> VEFNTDVLDAADKKNIDFTRFSEAGYVLPGQYLLDVIVNGQSISPASLQISFVEPQSSGDKAEKKLPQACLTSDMVRLMGLTAESLDKVVYWHDGQCADFHGLPGVDIRPDTGAGVLRINMPQARLEYSDATWLPPSRWDDGIPGLMLDYNLNGTVSRNYQGGDSHQFSYNGTVGGNLGPWRLRADYQGSQEQSRYNGEKTTNRNFTWSRFYLFRAIPRWRANLTLGENNINSDIFRSWSYTGASLESDDRMLPPRLRGYAPQITGIAETNARVVVSQQGRVLYDSMVPAGPFSIQDLDSSVRGRLDVEVIEQNGRKKTFQVDTASVPYLTRPGQVRYKLVSGRSRGYGHETEGPVFATGEASWGLSNQWSLYGGAVLAGDYNALAAGAGWDLGVPGTLSADITQSVARIEGERTFQGKSWRLSYSKRFDNADADITFAGYRFSERNYMTMEQYLNARYRNDYSSREKEMYTVTLNKNVADWNTSFNLQYSRQTYWDIRKTDYYTVSVNRYFNVFGLQGVAVGLSASRSKYLGRDNDSAYLRISVPLGTGTASYSGSMSNDRYVNMAGYTDTFNDGLDSYSLNAGLNSGGGLTSQRQINAYYSHRSPLANLSANIASLQKGYTSFGVSASGGATITGKDAALHAGGMSGGTRLLVDTDGVGGVPVDGGQVVTNRWGTGVVTDISSYYRNTTSVDLKRLPDDVEATRSVVESALTEGAIGYRKFSVLKGKRLFAILRLADGSQPPFGASVTSEKGRELGMVADEGLAWLSGVTPGETLSVNWDGKIQCQVNVPETAISDQQLLLPCTPQK;> AVSLDRTRAVFDGSEKSMTLDISNDNKQLPYLAQAWIENENQEKIITGPVIATPPVQRLEPGAKSMVRLSTTPDISKLPQDRESLFYFNLREIPPRSEKANVLQIALQTKIKLFYRPAAIKTRPNEVWQDQLILNKVSGGYRIENPTPYYVTVIGLGGSEKQAEEGEFETVMLSPRSEQTVKSANYNTPYLSYINDYGGRPVLSFICNGSRCSVKKEK;> MIRLSLFISLLLTSVTVLADVQINIRGHVYIPPCTINNGQNIVVDFGNINPEHVDNSRGEVTKTISISCPYKSGSLWIKVTGNTMGGGQNNVLATNITHFGIALYQGKGMSTPLTLGNGSGNGYRVTAGLDTARSTFTFTSVPFRNGSGILNGGDFRTTASMSMIYN;> MKKWFPALLFSLCVSGESSAWNNIVFYSLGDVNSYQGGNVVITQRPQFITSWRPGIATVTWNQCNGPGFADGFWAYYREYIAWVVFPKKVMTQNGYPLFIEVHNKGSWSEENTGDNDSYFFLKGYKWDERAFDAGNLCQKPGETTRLTEKFDDIIFKVALPADLPLGDYSVKIPYTSGMQRHFASYLGARFKIPYNVAKTLPRENEMLFLFKNIGGCRPSAQSLEIKHGDLSINSANNHYAAQTLSVSCDVPANIRFMLLRNTTPTYSHGKKFSVGLGHGWDSIVSVNGVDTGETTMRW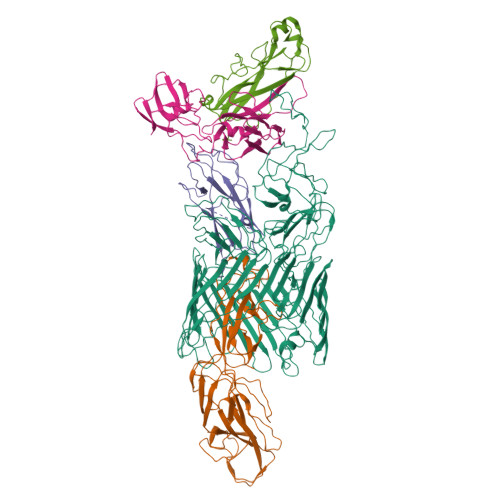YKAGTQNLTIGSRLYGESSKIQPGVLSGSATLLMILP;> MIKSTGALLLFAALSAGQAIASDVAFRGNLLDRPCHVSGDSLNKHVVFKTRASRDFWYPPGRSPTESFVIRLENCHATAVGKIVTLTFKGTEEAALPGHLKVTGVNAGRLGIALLDTDGSSLLKPGTSHNKGQGEKVTGNSLELPFGAYVVATPEALRTKSVVPGDYEATATFELTYR> MERTELLK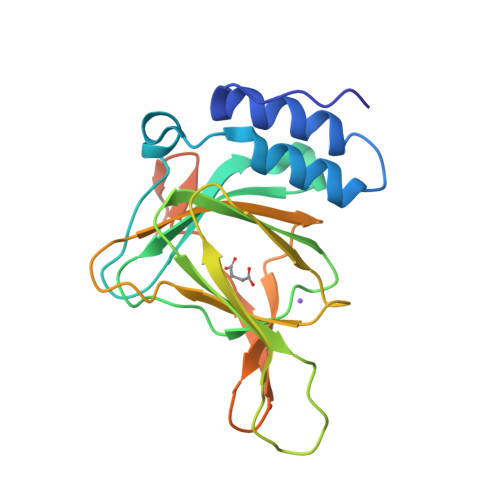PRTLADLIRILHELFAGDEVNVEEVQAVLEAYESNPAEWALYAKFDQYRYTRNLVDQGNGKFNLMILCWGEGHGSSIHDHTDSHCFLKLLQGNLKETLFDWPDKKSNEMIKKSERTLRENQCAYINDSIGLHRVENVSHTEPAVSLHLYSPPFDTCHAFDQRTGHKNKVTMTFHSKFGIRTPFTTSGSLENNSAWSHPQFEK> RTSTIMTDYNPNYSFAGKTSSISDLKEVPRKNITLIRGLGHGAFGEVYEGQVSGMPNDPSPLQVAVKTLPEVCSEQDELDFLMEALIISKFNHQNIVRCIGVSLQSLPRFILLELMAGGDLKSFLRETRPRPSQPSSLAMLDLLHVARDIACGCQYLEENHFIHRDIAARNCLLTCPGPGRVAKIGDFGMAQDIYRASYY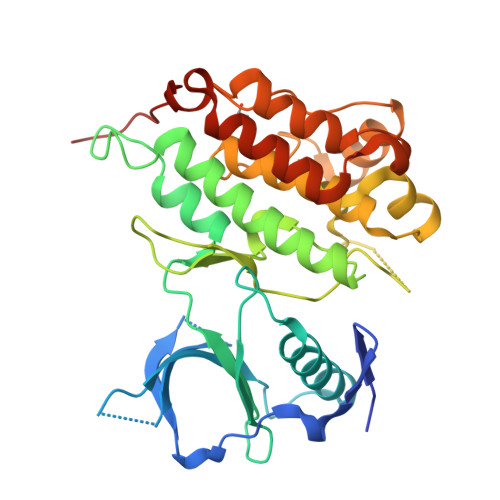RKGGCAMLPVKWMPPEAFMEGIFTSKTDTWSFGVLLWEIFSLGYMPYPSKSNQEVLEFVTSGGRMDPPKNCPGPVYRIMTQCWQHQPEDRPNFAIILERIEYCTQDPDVINTALPIEYGPLVEEEEK> VTVVEEVDHLPIYDLDPKLEEFKDHFNYRIKRYLDQKCMIEKHEGGLEEFSKGYLKFGINTVDGATIYREWAPAAQEAQLIGEFNNWNGAKHKMEKDKFGIWSIKISHVNGKPAIPHNSKVKFRFRHGGGAWVDRIPAWIRYATFDASKFGAPYDGVHWDPPACERYVFKHPRPPKPDAPRIYEAHVGMSGEEPEVSTYREFADNVLPRIRANNYNTVQLMAIMEHSYYASFGYHVTNFFAVSSRSGTPEDLKYLVDKAHSLGLRVLMDVVHSHASNNMTDGLNGYDVGQNTHESYFHTGDRGYHKLWDSRLFNYANWEVLRFLLSNLRYWMDEFMFDGFRFDGVTSMLYHHHGINKGFTGNYKEYFSLDTDVDAIVYMMLANHLMHKLLPEATIVAEDVSGMPVLCRPVDEGGVGFDFRLAMAIPDRWIDYLKNKEDRKWPMSEIVQTLTNRRYTEKCIAYAESHDQSIVGDKTIAFLLMDKEMYTGMSDLQPASPTINRGIA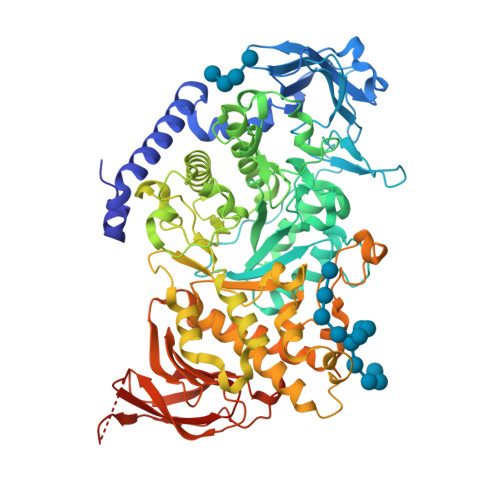LQKMIHFITMALGGDGYLNFMGNEFGHPEWIDFPREGNNWSYDKCRRQWSLVDTDHLRYKYMNAFDQAMNALEEEFSFLSSSKQIVSDMNEKDKVIVFERGDLVFVFNFHPNKTYKGYKVGCDLPGKYRVALDSDALVFGGHGRVGHDVDHFTSPEGMPGVPEANFNNRPNSFKVLSPPRTCVAYYRVDEDREELRR> IVGGQECKDGECPWQALLINEENEGFCGGTILSEFYILTAAHCLYQAKRFKVRVGDRNTEQEEGGEAVHEVEVVIKHNRFTKETYDFDIAVLRLKTPITFRMNVAPACLPERDWAESTLMTQKTGIVSGFGRTHEKGRQSTRLKMLEVPYVDRNSCKLSSSFIITQNMFCAGYDTKQEDACQGDSGGPHVTR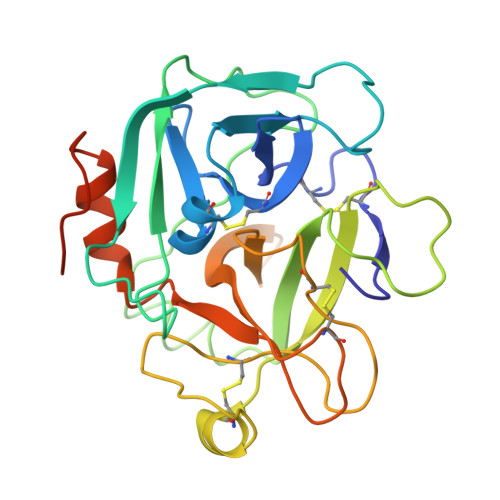FKDTYFVTGIVSWGEGCARKGKYGIYTKVTAFLKWIDRSMKTRGLPKAKSHAPEVVITSSPLK N-[(E)-iminomethyl]-L-aspartic 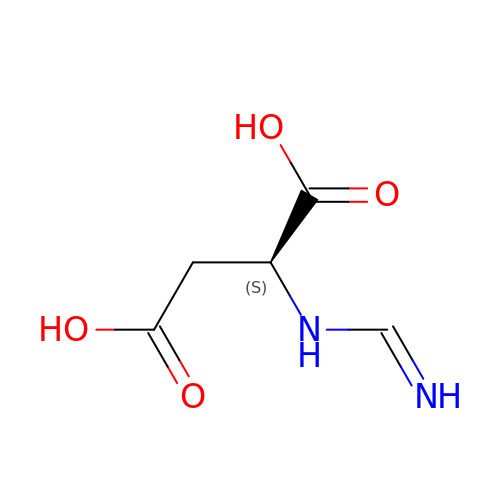acid | C5 H8 N2 O4 | XTPIFIMCFHNJOH-VKHMYHEASA-N> GASGRGEAETRECIYYNANWELERT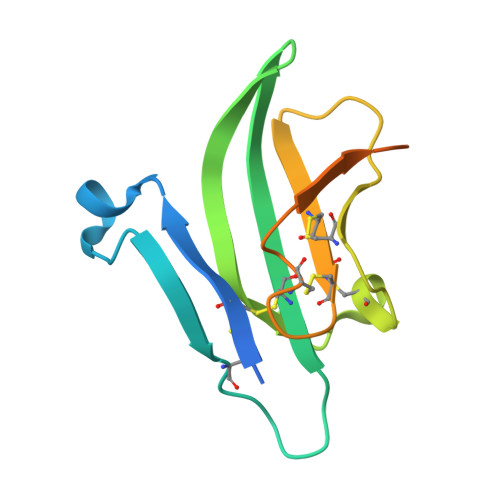NQSGLERCEGEQDKRLHCYASWRNSSGTIELVKKGCWLDDFNCYDRQECVATEENPQVYFCCCEGNFCNERFTHLPEAGGPEVTYEPPPTAPTGDDDDK> MSQNNPLRALLDKQDILLLDGAMATELEARGCNLADSLWSAKVLVENPELIREVHLDYYRAGAQCAITASYQATPAGFAARGLDEAQSKALIGKSVEL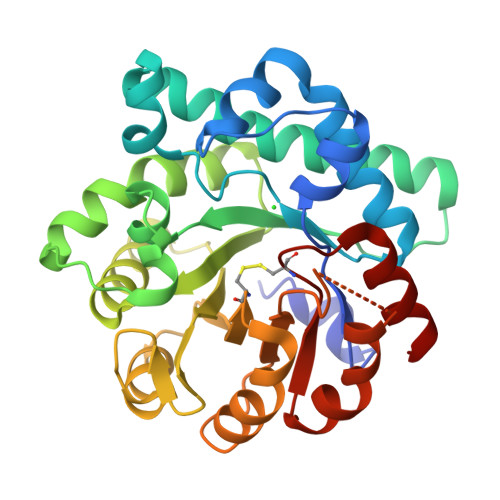ARKAREAYLAENPQAGTLLVAGSVGPYGAYLADGSEYRGDYHCSVEAFQAFHRPRVEALLDAGADLLACETLPNFSEIEALAELLTAYPRARAWFSFTLRDSEHLSDGTPLRDVVALLAGYPQVVALGINCIALENTTAALQHLHGLTVLPLVVYPNSGEHYDAVSKTWHHHGEHCAQLADYLPQWQAAGARLIGGCCRTTPADIAALKARS3-azanyl-5-[(2~{S})-3-methylbutan-2-yl]-7-[1-methyl-5-(2-oxidanylpropan-2-yl)pyrazol-3-yl]-1~{H}-pyrazolo[4,3-c]pyridin-4-one 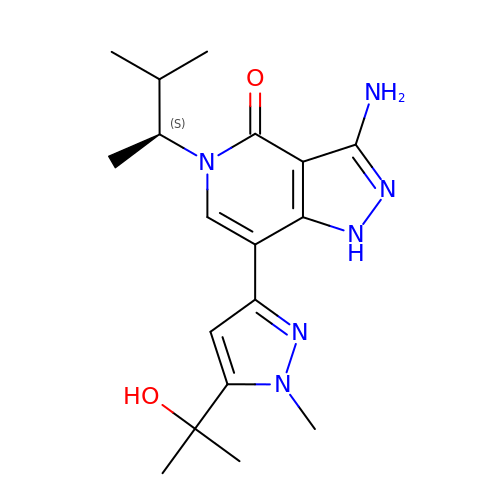| C18 H26 N6 O2 | MUDVASGRHKWSTJ-JTQLQIEISA-N(4R)-4-methyl-1,3,4,5-tetrahydro-2H-1,5-benzodiazepin-2-one 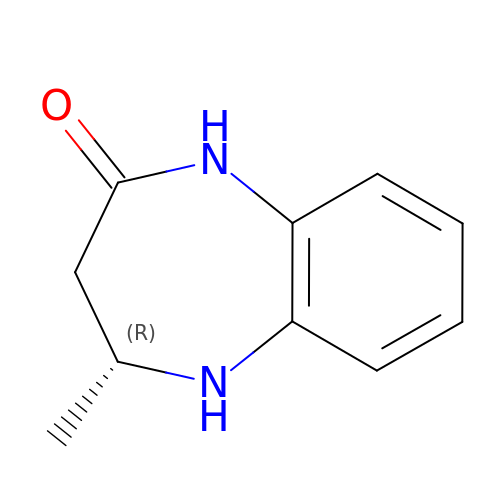| C10 H12 N2 O | BBPWQLMHOSRDMA-SSDOTTSWSA-N>[2x]CAGUGG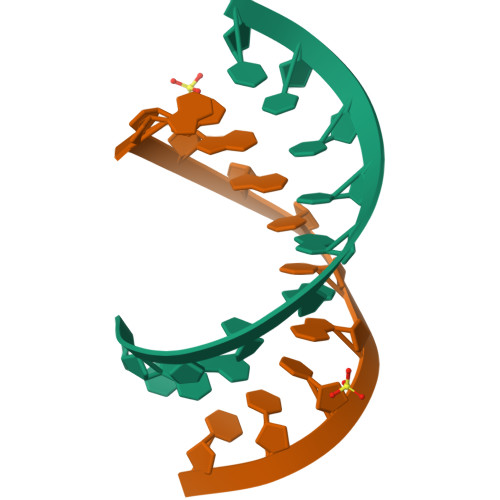UCUU;>AAGACUGCCUG[2x]>MRA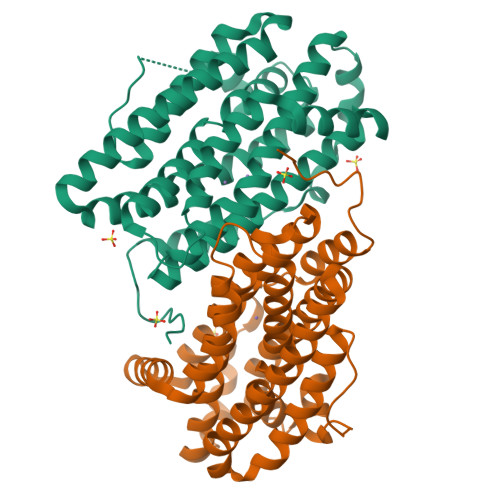VNWNKKEDDFSLMFWKQNIAQFWTEEEIAVSSDKNTWVQLSKEEQIAYKRVLGGLTLLDTKQGGEGMPLVLVHLENLQAKSVLAFMGAMEEVHAKSYSHIFTTLATEEEIDEIFDWVDTHPLLEKKAGIITSYYRRLLKPEVTKKELYMAMVASVFLESYLFYSGFFYPLYLAGQGKLTASGEIINLIIRDESIHGVFVGILAQQIFAELSAEDQQEVQKETQELLMELYEIEMAYTEEIYTSIGLVEDVNRFVRYNANKGLMNLGLEPKFEEEEINPIVLNGLRTDTKNHDFFSVKGNGYVKATNVEKLSDDDFVFNF[2x]>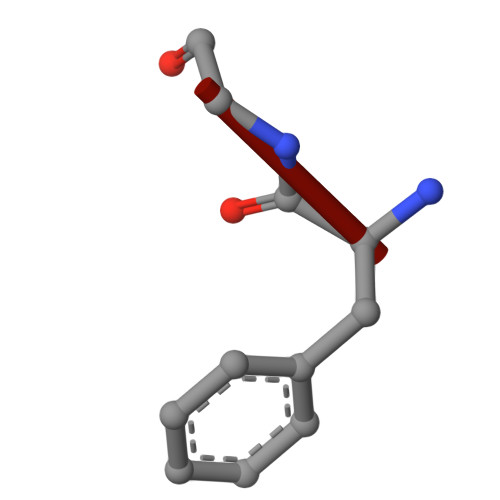 FG>[2x]TADAVLMIEANLDDQTGEGLGYVMNQLLTAGAYD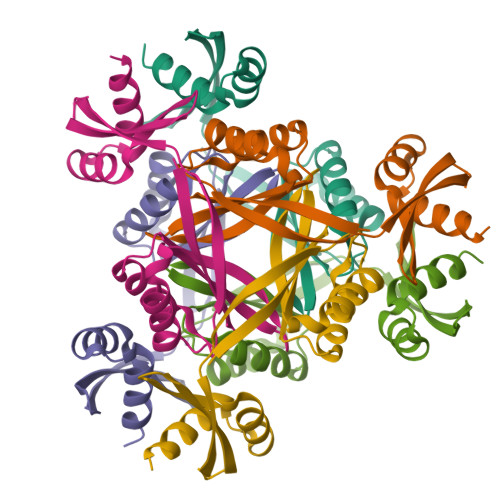VFFTPIQMKKDRPATKLTVLGNVNDKDLLTKLILQETTTIGVRYQTWQRTIMQRHFLTVATPYGDVQVKVATYQDIEKKMPEYADCAQLAQQFHIPFRTVYQAALVAVDQLDEEA> GSTLVTGSEYETMLTEIMSMGYERERVVAALRASGNNPH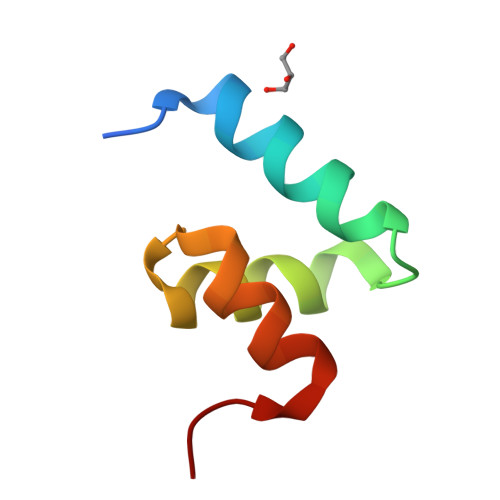RAVEYLLTGIPG> MQRVVVAIDAKRVDGEFMVFTHSGKKNTGILLRDWVVEVEKRGAGEILLTSIDRDGTKSGYDTEMIRFVRPLTTLPII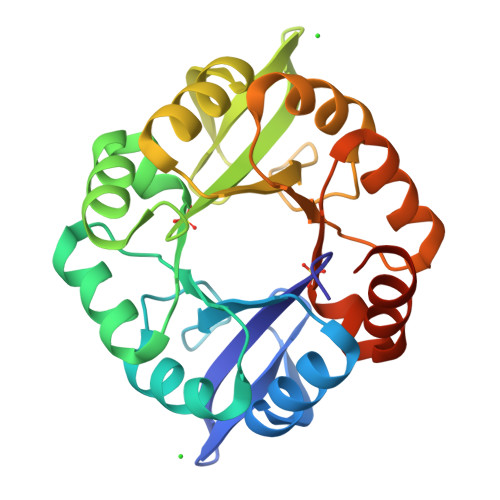ASGGAGKMEHFLEAFLAGADKVSINTAAVENPSLITQIAQTFGSQAVVVAIDAKRVDGEFMVFTHSGKKNTGILLRDWVVEVEKRGAGEILLTSIDRDGTKSGYDTEMIRFVRPLTTLPIIASGGAGKMEHFLEAFLAGADKVSINTAAVENPSLITQIAQTFGSLEHHHHHH>MAAALSEQLAELEKRSGGRLGVAVLDTATGRRFGYRGDERFPMCSTFKALLA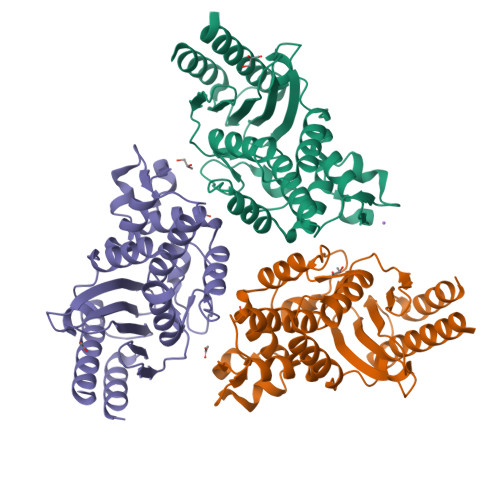AAVLARVDQGKENLDRRITYGKEDLVDYSPVTEKHVGDGMTVAELCEAAITYSDNTAANLLLEALGGPAALTAFLRSIGDNVTRLDRWEPELNTAAPGDPRDTTTPAAMAATLRTLLLGDVLSPASRQQLVDWLIANKTGDKRLRAGLPADDRVGDKTGTGEHGTTNDIAVVWPPNHAPIFLAVYLTESQVDADARDAVIAEVARLVVAAWVHHHHH[3x]> MLLQKEREEIVAYGKKMISSGLTKGTGGNISIFNREQGLVAISPSGLEYYETKPEDVVILNLDGEVIEGERKPSSELDMHLIYYRKREDINALVHTHSPYAKTIASLGWELPAVSYLIAFAGPNVRCAPYETFGTKQLADAAFEGMIDRRAVLLANHGLIAGANNIKMAFTVAEEIEFCAQIYYQTKSIGEPKLLPEDEMENLAKKFEGYGQQYLEHHHHHH

Here we demonstrate a dAdo disposal and salvage pathway leading via 5-deoxyribose, dR1P, and dRu1P to the mainstream metabolites acetaldehyde and DHAP. The three enzymes, acting together in the presence of ATP, were necessary and sufficient to generate DHAP from 5-deoxyribose, as shown by using a coupled assay to measure DHAP formation. This result fits with the predicted reaction sequence in which the kinase mediates ATP-dependent 1-phosphorylation of 5-deoxyribose, the isomerase converts dR1P to dRu1P, and the aldolase cleaves dRu1P to acetaldehyde and DHAP. DrdA is a unique member of the class II aldolase family of enzymes, differing from most others in both the nature of the metal (Mn2+) and the aldehyde co-substrate. Although, like similar aldolases, DrdA is promiscuous with respect to the aldehyde co-substrate, it is unusual in preferring acetaldehyde.

Our two structures of DrdA, bound and unbound with substrate, along with previous data on class II aldolases, allow a detailed mechanistic proposal. A structural homology search showed most significant homology to fuculose 1-phosphate aldolase, solved from various organisms, with homology to the E. coli enzyme the strongest. Structures of fuculose-1-phosphate aldolase (FucA) determined from several sources including S. pneumoniae and E. coli exhibit a fold common to the class II aldolase family composed of a five-stranded antiparallel β-sheet core surrounded by eight α-helices of varying length. The metal coordination around Mn2+ is close to ideal tetrahedral in the apo-structure and is a distorted trigonal bipyramid in the complexed structure. Without a supplement, zinc is the predominant metal found in the enzyme, however with an excess of metals included, manganese is incorporated at a higher percentage. These results are consistent with manganese being the preferred cofactor when low abundancy is excluded. The addition of Mn2+ to demetallated DrdA resulted in higher aldolase activity than addition of Co2+, Mg2+, Ni2+, or Zn2+; the apparent Kmetal value for Mn2+ was 0.95 ± 0.31 µM (mean and s.d. of three determinations).> MTGIPTVTARPWTQRPRAENSTTNPTYFFTFGDXYSQ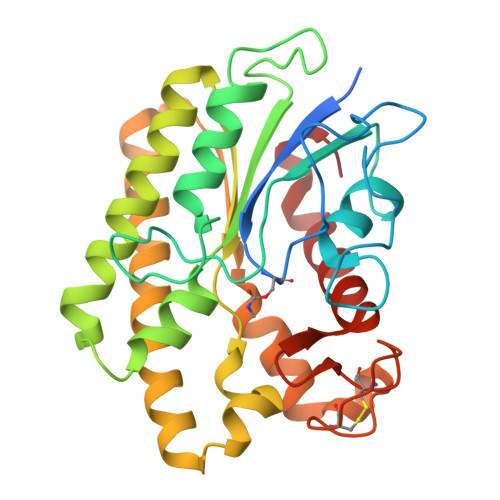TGFSASGTQPSASNPMGNPDLGIGTTTNGPNWIGYLTTTENASLVLSYNLAAGGATIDNALVPAYPGDLASQFRLFEDVYADKPASAPWSAEDAVFGVWIGINDIGNAYYSTDAETYTPKLISRLESLVEEVYKNGGRKFLFLNVPPTSRSPLFLEQGEEVVKQHAEYLSVYNENLEGMVDDFTKKKGDVTTVLYDSWSFMTKILDDPTAYGFPDATCINDDGTSCIWWNNYHPGMKYHLLQAEDMKPKLRKLGGW>DYKDDDDKHHHHHHHHHHLEVLFQGPQSSERRVVAHMPGDIIIGALFSVHHQPTVDKVHERKCGAVREQYGIQRVEAMLHTLERINSDPTLLPNITLGCEIRDSCWHSAVALEQSIEFIRDSLISSEEEEGLVRCVDGSSSSFRSKKPIVGVIGPGSSSVAIQVQNLLQLFNIPQIAYSATSMDLSDKTLFKYFMRVVPSDAQQARAMVDIVKRYNWTYVSAVHTEGNYGESGMEAFKDMSAKEGICIAHSYKIYSNAGEQSFDKLLKKLTSHLPKARVVACFCEGMTVRGLLMAMRRLGLAGEFLLLGSDGWADRYDVTDGYQREAVGGITIKLQSPDVKWFDDYYLKLRPETNLRNPWFQEFWQHRFQCRLEGFPQENSKYNKTCNSSLTLKTHHVQDSKMGFVINAIYSMAYGLHNMQMSLCPGYAGLCDAMKPIDGRKLLESLMKTAFTGVSGDTILFDENGDSPGRYEIMNFKEMGKDYFDYINVGSWDNGELKMDDDEVWSKKSNIIRSVCSEPCEKGQIKVIRKGEVSCCWTCTPCKENEYVFDEYTCKACQLGSWPTDDLTGCDLIPVQYLRWGDPEPIAAVVFACLGLLATLFVTVVFIIYRDTPVVKSSSRELCYIIL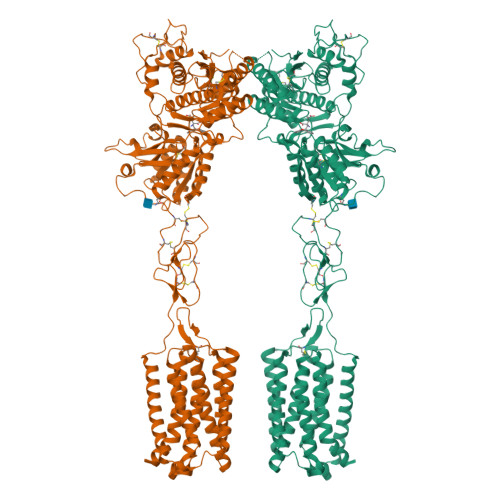AGICLGYLCTFCLIAKPKQIYCYLQRIGIGLSPAMSYSALVTKTNRIARILAGSKKKICTKKPRFMSACAQLVIAFILICIQLGIIVALFIMEPPDIMHDYPSIREVYLICNTTNLGVVAPLGYNGLLILACTFYAFKTRNVPANFNEAKYIAFAMYTTCIIWLAFVPIYFGSNYKAITMCFSVSLSATVLLGCMFVPKVYIILAKPERNVRSAFTTSTVVRMHVGDGKSSSAA[2x]ACETYL 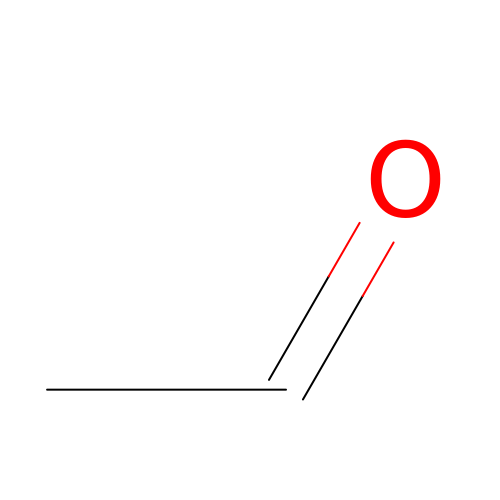GROUP | C2 H4 O | IKHGUXGNUITLKF-UHFFFAOYSA-N> XCAIDQDFLDAAGILENEA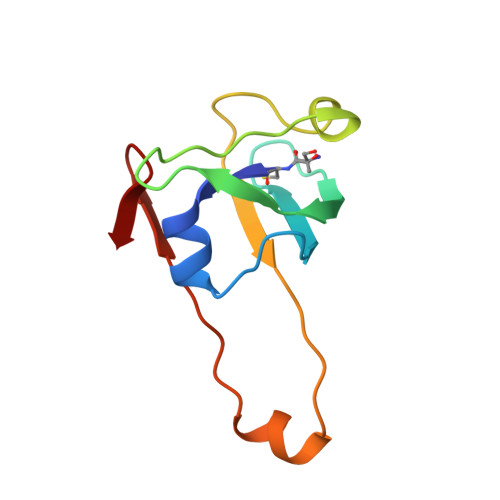IDIWNVTNGKRFSTYAIAAERGSRIISVNGAAAHCASVGDIVIIASFVTMPDEEARTWRPNVAYFEGDNEMK> MGMPVPGTLSVEIPPRYCPLPTARHPDETVLARRTADWIDGFDLELTPQQRARMRGNDCPGFYGRIMPHSPTDRLQLAVDWCTVMFHFDDVHCDEGPATGRAARFADLATRIVRVLEAPDARLEGPGDTMLAPVRDLALRARRWATPAQMRRCAEAHRAWFLAVAWELGHRAARSTPALNDYAHMRQHTAAGAATLAWAEIVDGAEIPDRELSSPEVRALTELAFTTAAFDDDLFSYGKELWVARAEGTAPSGLGLVEILRRENRCGRPEALRAAVCLCNRLTHRFIALRERVLPDASAPLRAYLDHLCHLLPGNLEWGLTADRYRNPDGRTPGAVTTTASRDTDPPADTSPPAIPSIAWWWDPLGGRPATEHHHHHH

We recently discovered the cattleyene synthase (CyS) from Streptomyces cattleya and studied its cyclization mechanism through isotopic labelings. Some polycyclic diterpenoids have attracted increasing attention, e.g. gibberellins are phytohormones derived from ent‐kaurene, while phorbol esters exhibiting the tigliane skeleton are currently in phase II clinical trials for the treatment of acute myeloid leukemia. Their biosynthesis is attributed to diterpene synthases (DTSs), the type I of which catalyzes the conversion of GGPP through diphosphate abstraction and cationic cascade reactions. Substrate ionization is mediated by a Lewis acidic trinuclear Mg2+ cluster, bound itself to a highly conserved Asp‐rich motif (DDXX(X)D) and an NSE/DTE triad ((N,D)DLX(S,T)XXXE), to which the substrate's pyrophosphate docks, with assistance of a highly conserved Arg residue (pyrophosphate sensor). Here we report on the crystal structures of apo‐CyS, CyS complexed with GGPP and Mg2+ (CyS‐GGPP‐Mg2+), and the CySC59A enzyme variant.

Apo‐CyS adopts the classical α‐helical fold of class I TSs, with ten core (A‐J) and three short α helices (α1–α3). The Asp‐rich motif (D89DVHCD94) is located on helix C and the NSE triad (D232DLFS236YGKE240) on helix H. The CyS‐GGPP‐Mg2+ structure shows a similar fold to apo‐CyS, with a root‐mean‐square deviation (RMSD) of 0.24 Å for Cα atoms. Upon GGPP and Mg2+ binding one more α helix (α4) and two β strands (β1 and β2) close to the active site become ordered. In the apo‐CyS and CyS‐GGPP‐Mg2+ structures, the thiol of C59 is close to the phenyl ring of F86 (3.4 Å) and renders it towards the active site, while in CySC59A this interaction is disrupted.>MDWRHKAVCRDEDPELFFPVGNSGPALAQIADAKLVCNRCPVTTECLSWALNTGQDSGVWGGMSEDERRALKRRNA[2x];>[2x]MAHHHHHHAREPISLDQTIGDEGDSQLGDFIEDSEAVVAVDAVSFTLLQDQLQSVLDTLSEREAG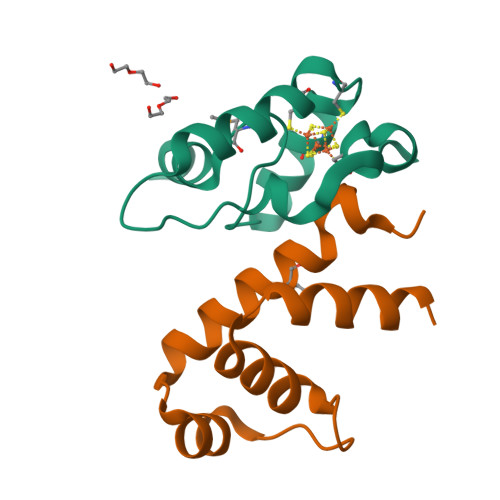VVRLRFGLTDGQPRTLDEIGQVYGVTRERIRQIESKTMSKLRHPSRSQVLRDYLD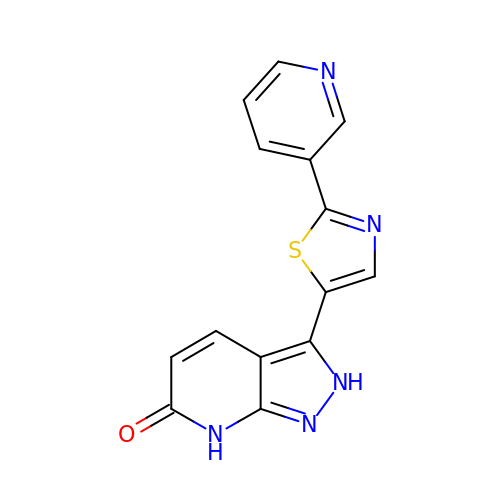3-[2-(pyridin-3-yl)-1,3-thiazol-5-yl]-2,7-dihydro-6H-pyrazolo[3,4-b]pyridin-6-one | C14 H9 N5 O S | JCIZDZAGSUATFA-UHFFFAOYSA-N>CPSRCSCSGTEIRCNSKGLTSVPTGIPSSATRLELESNKLQSLPHGVFDKLTQLTKLSLSSNGLSFKGCCSQSDFGTTSLKYLDLSFNGVITMSSNFLGLEQLEHLDFQHSNLKQMSEFSVFLSLRNLIYLDISHTHTRVAFNGIFNGLSSLEVLKMAGNSFQENFLPDIFTELRNLTFLDLSQCQLEQLSPTAFNSLSSLQVLNMSHNNFFSLDTFPYKCLNSLQV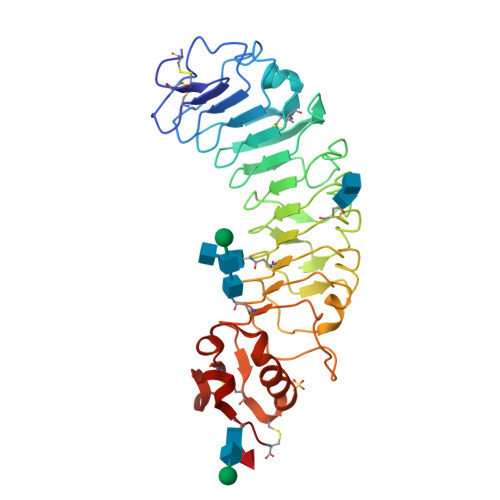LDYSLNHIMTSKKQELQHFPSSLAFLNLTQNDFACTCEHQSFLQWIKDQRQLLVEVERMECATPSDKQGMPVLSLNITC[4x]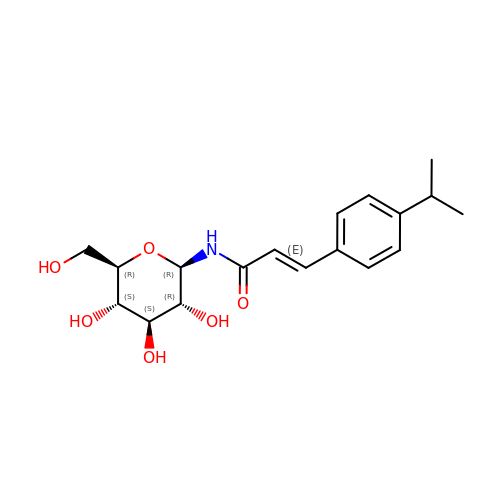N-{(2E)-3-[4-(propan-2-yl)phenyl]prop-2-enoyl}-beta-D-glucopyranosylamine | C18 H25 N O6 | OPYZIUIJGFRFFX-AWRGUQPNSA-N> PTTENLYFQGAMALEEIKNGTDISTLDIRKFNLNINNVSVLSKSQSVDQFHLSNPHYEYLSGGAYPGEMENFTLKVDKSKKQDQVFENPLSLKFTNIGTVNGKQVDAYLNFNKVTLHYLNTAQAESEMNSAQKSTVEFFSISELWESNAFEIGNVPYVDANHDYIMNKAFWIDADVTAEIRYADGTETDLKLVMKPTDIDAIDANNLKETFYVKNYQNDVNLRLMNNANVLVQEEASDRTSWIATQITGGSYNENNVSGLALRSNSNSMNFGYSSTETCSAVFGLYIE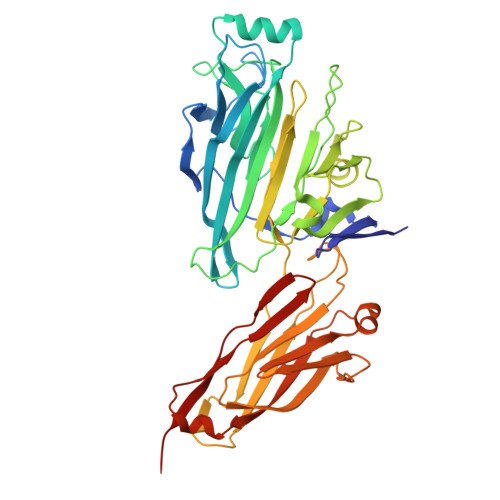KIDPRPVLEVDPAEIPAKDGQDVTYKATFKVPVPGKDILAAPSSIEMVQKFDERLDYKELKVESGGVTLQEGRDYTIEKTGQTVTVKMTPEYLKGNSSSDIIITYKTATNKKVEEKGSEKIDNTVTLHVDNLSAPSNQVSTALLYEK> MSKHCGLEANQKATDNEPKKRIRWNKSQRTLIEKLTADKHRKLRQSRRTADIYGDEVSAAQSQKLAEIEEVLIRSAGDVISLDRGQYDKWASLVSAKLGWRRGNPLNPSLNYSQAGEVREALKDARRVAQNLINDASHIRMLDGIKRFDDIYR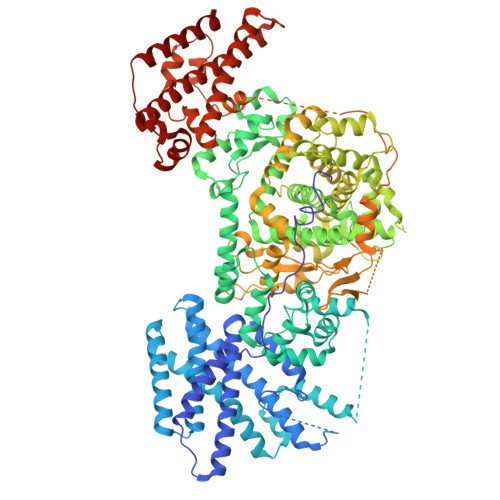QIMKPLGMTTDDARALFNETIEIGSIPKNNKIYGNSEGVRLINSLRHSDYIERAKGYGLNDEAIETLLRAATDVHSVFDEMRVIAEATGHNIEELQNLGYFPRIATRDFNIRLRKALETDTALADVIMSEGVEQVKALNPLSSVWQKSRKFNYFVPDDLEVASKLLNTSSDEIAEMLLNPREWMEFLTSSVSSSQIETMTELGVMSKLPMTSREVFEQLVDQYELPYKHINEMFKLDPHVAAEEYARVLRQAVGNSAMLKTVVKDGLAAGWAVPEKMLKDLSPKERANFVPLSFQKLDQFMSPEQLEAAGKVYVHRVVSDQWRSMLEISMSANKLGAFASAWSHLSTFLNKSVLASRNVLYVGTNFLSGFVLTNAVGANVFTVPHAMMDISNYLAKGLDAFDGTKPFAKIGGEWISKREFFKQFLLKRGSDITPGTVSTTSSGGDANPFTSFKSIGALADVRSAKRALEYLWSYSSSFGDPVRGTKGAAEYVGSLLNEATDNFFSPFAKMASFLDTMYKWNAYTSLVERQGAAELANTIAQGMTLEPISRIGRKFDNWRDLSRHIDDYFFTFDDPGTTTKVISKYVRPFANWSMQSTPAMLRAALRSPQKFSAYAKLLQLYNRGNNDDEPLNQSQLTDWQDDEYPVILQRDALQTGDGNGGLLVLFPHTFDPITDTLNVIDNAGRTVNILFGNKYGGNERDNRNSVTGKKDGLTSMLTELFNDTYWAKPAGLLLGIDSFTGQKIDASKYNNYLGFEMHPLAEALLGMYTPLDAINRTNLFDTFGRREYKDYRDRTVVEEKPGLFGGQRTNSDAQSLAWETAVKNGNWSALALMTMGARVRLIDTARNTQMTLDEIKTGIDELQKANVNAARQLTLNPEKLSESERNKRTERLTESLTAEYQMKYDYARLINYMKAKRIPPKRLLFEMQQRSVNVSDLEPVGGKQRLQLESDFRRRIEEINK> DDDDEEEDDFVYFNFNKEKEEKNKNSIHPNDFQIYNSLKYKYHPEYQYLNIIYDIMMNGNKQSDRTGVGVLSKFGYIMKFDLSQYFPLLTTKKLFLRGIIEELLWFIRGETNGNTLLNKNVRIWEANGTREFLDNRKLFHREVNDLGPIYGFQWRHFGAEYTNMYDNYENKGVDQLKNIINLIKNDPTSRRILLCAWNVKDLDQMALPPCHILCQFYVFDGKLSCIMYQRSCDLGLGVPFNIASYSIFTHMIAQVCN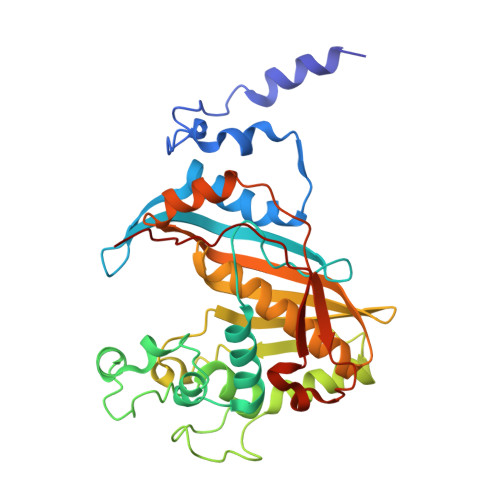LQPAQFIHVLGNAHVYNNHIDSLKIQLNRIPYPFPTLKLNPDIKNIEDFTISDFTIQNYVHHEKISMDMAA> MVTFHTNHGDIVIKTFDDKAPETVKNFLDYCREGFYNNTIFHRVINGFMIQGGGFEPGMKQKATKEPIKNEANNGLKNTRGTLAMARTQAPHSATAQFFINVVDNDFLNFSGESLQGWGYCVFAEVVDGMDVVDKIKGVATGRSGM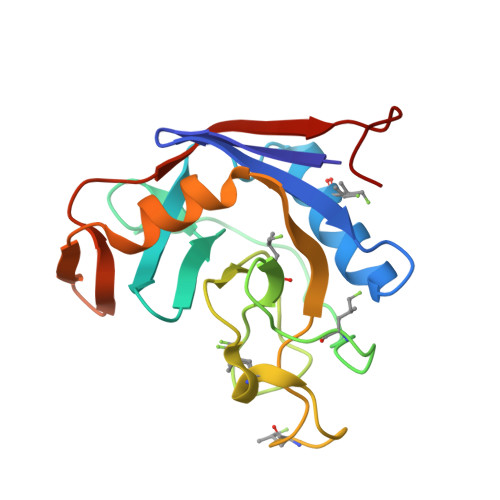HQDVPKEDVIIESVTVSEHHHHHH>[4x]SLIENSHVKKDDIWPSGGQMTVKDLTAKYTEGGNAILENISFSISPGQRVGLLGRTGSGKSTLLSAFLRLLNTEGEIQIDGVSWDSITLEQWRKAFGVIPQKVFIFSGTFRKNLDPNAAHSDQEIWKVADEVGLRSVIEQFPGKLDFVLVDGGCVLSHGHKQLMCLARSVLSKAKILLLDEPSAHLDPVTYQIIRRTLKQAFADCTVILCEARIEAMLECDQFLVIEEN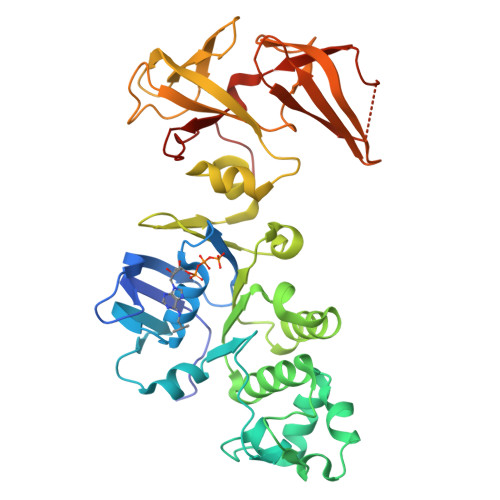KVRQYDSILELYHYPADRFVAGFIGSPKMNFLPVKVTATAIDQVQVELPMPNRQQVWLPVESRDVQVGANMSLGIRPEHLLPSDIADVILEGEVQVVEQLGNETQIHIQIPSIRQNLVYRQNDVVLVEEGATFAIGLPPERCHLFREDGTACRRLHKEPGV> GAMDHVEFGLTYSQLMTLKDAMLQLDPNAKTWMDIEGRPEDPVEIALYQPSSGCYIHFFREPTDLKQFKQDAKYSHGIDVTDLFATQPGLTSAVIDALPRNMVITCQGSDDIRKLLESQGRKDIKLIDIALSKTDSRKYE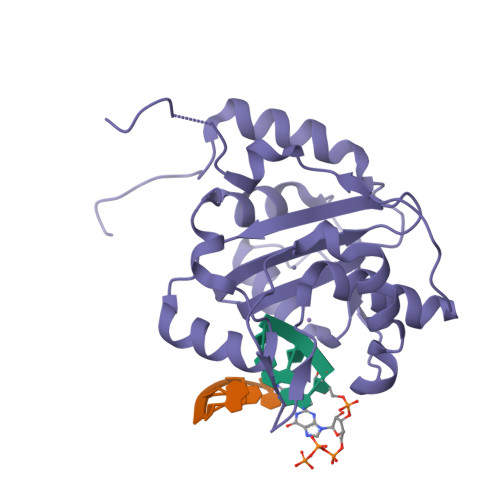NAVWDQYKDLCHMHTGVVVEKKKRGGKEEITPHCALMDCIMFDAAVSGGLNTSVLRAVLPRDMVFRTSTPRVVL>MSKEYHIDEEVGFALPNPQENLPDFYNDWMFIAKHLPDLIESGQLRERVEKLNMLSIDHLTDHKSQRLARLVLGCITMAYVWGKGHGDVRKVLPRNIAVPYCQLSKKLELPPILVYADCVLANWKKKDPNKPLTYENMDVLFSFRDGDCSKGFFLVSLLVEIAAASAIKVIPTVFKAMQMQERDTLLKALLEIASCLEKALQVFHQIHDHVNPKAFFSVLRIYLSGWKGNPQLSDGLVYEGFWEDPKEFAGGSAGQSSVGQCFDVLLGIQQTAGGGHAAQFLQDMRRYMPPAHRNFLCSLESNPSVREFVLSKGDAGLREAYDACVKALVSLRSYHLQIVTKYILIPASQQPKENKTSEDPSKLEAKGTGGTDLMNFLKTVRSTTEKSLLKEGKGELNSKLEGKPIPNP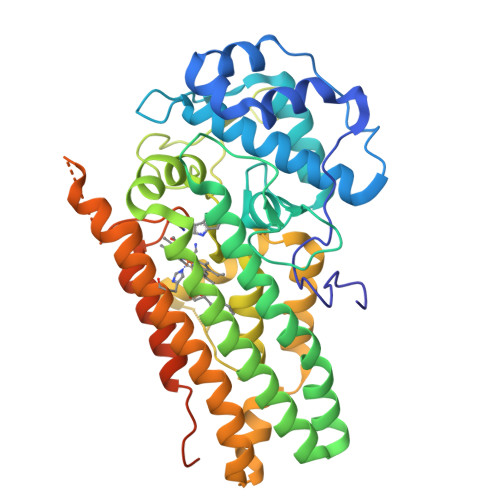LLGLDSTRTGHHHHHH[2x]>GSMNKHTEHDTREHLLATGEQLSLQRGFTGMGLSELLKTAEVPKGSFYHYFRSKEAFGVAMLERHYAAYHQRLTELLQSGEGNYRDRILAYYQQTLNQFSQHGTISGCLTVKLSAEVSDLSEDMRSAMDKGARGVIALLSQALENGRENHSLTFSGEP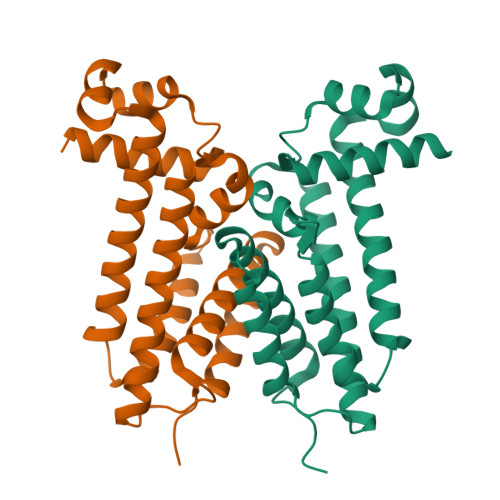LQQAQVLYALWLGANLQAKISRSFEPLENALAHVKNIIATPAV[4x]> MGSSHHHHHHHSSENLYFQGLIDRGQDLADVAKYPLITGFFRIEMNVVRLDTQGKSHTGLPCDIFDKCDPKIIAFIDTEKPNNDFGGDSVPYSNYITLVDANNTPDVVEIDKTISRDVCGKGVRKIAMRVRAIDKDGLNDDKIDNYKCHITGERNPPAENEKVAQWSPEIACAGEDRASSKVYLRYRWYNIPESTCRPSSNGQGLFSGLF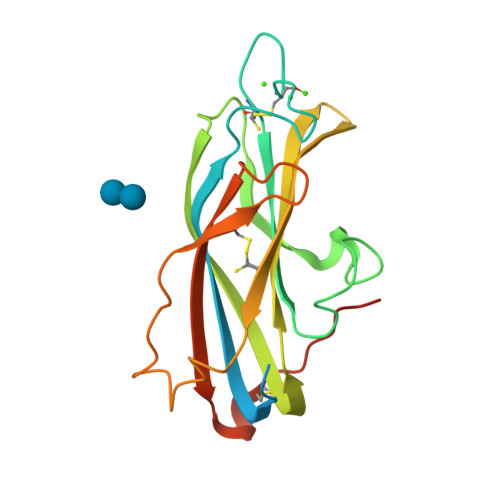SR> MTVEAFHKMENMKPKDYKSEVPTTWCPGCGHFGILNGVYRAMAELGIDSTKFAAISGIGCSSRMPYFVDSYKMHTLHGRAGAVATGTQVARPDLCVVVAGGDGDGFSIGGGHMPHMARKNVNMTYVLMDNGIYGLTKGQYSPTSRPEMTAYTTPYGGPENPMNPLLYMLTYGATYVAQAFAG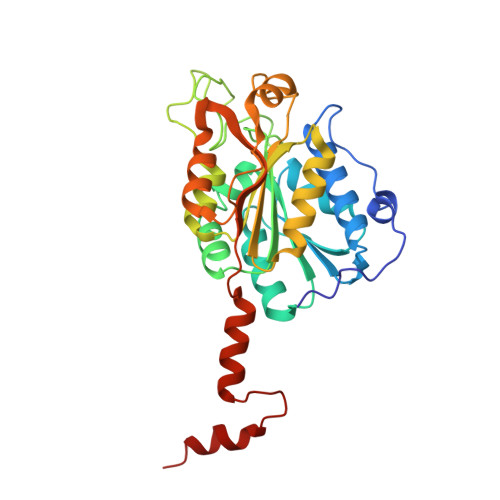KPKDCAELIKGAMEHEGFAYVNIFSQCPTFNKIDTVDFYRDLVEPIPEDHDTSDLGAAMELARRPGGKAPTGLLYKTSAPTLDQNLAKIRERLGGHVGYDKNKIIALAKP>MLETRATTAKQLVQAPEQPAPQPEVAPPTTEQPAPAPAPGTTPGTENFNTPNATPETTEPRVLVSEVLVRPQSGQLTPELETQVYNVIRTQPGRTTTRSQLQEDINAIFGTGFFSNVQASPEDTPLGVRVSFIVQPNPVLSKVE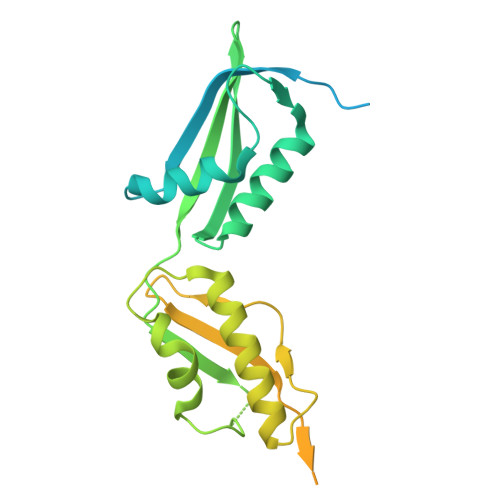IQANPGTNVPSVLPQATADEIFRAQYGKILNLRDLQEGIKELTKRYQDQGYVLANVVGAPQVSENGVVTLQVAEGVVENISVRFRNKEGQDVNEQGQPIRGRTQDYIITREVELKPGQVFNRNTVQKDLQRVFGTGLFEDVNVSLDPGTDPTKVNVVVNVVERSLEHHHHHH[2x]>[2x]GAMKDEWTGLVEQADPPIRAKAAEIAVAHAHYLSIEFYRIVRIDPHAEEFLSNEQVERQLKSAMERWIINVLSAQV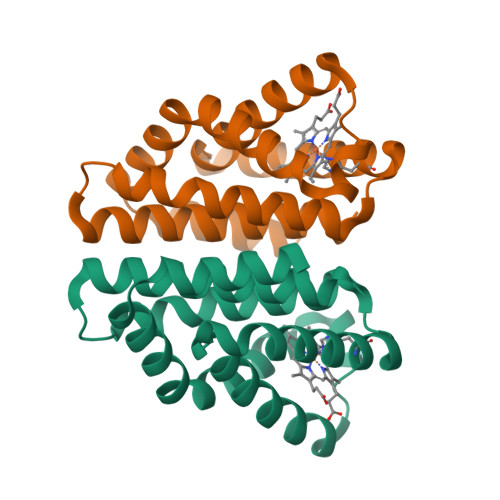DDVERLIQIQHTVAEVHARIGIPVEIVEMGFRVLKKILYPVIFSSDYSAAEKLQVYHFSINSIDIAMEVMTRAFTFSDSSASKEDENYR> MAEGNTLISVDYEIFGKVQGVFFRKHTQAEGKKLGLVGWVQNTDRGTVQGQLQGPISKVRHMQEWLETRGSPKSHID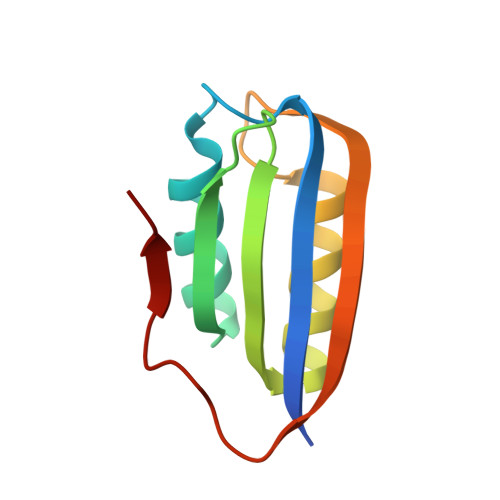KANFNNEKVILKLDYSDFQIVK>SMKPRCLHLEKGPQGFGFLLREEKGLDGRPGQFLWEVDPGLPAKKAGMQAGDRLVAVAGESVEGLGHEETVSRIQGQGSCVSLTVVDPEADRETSV[6x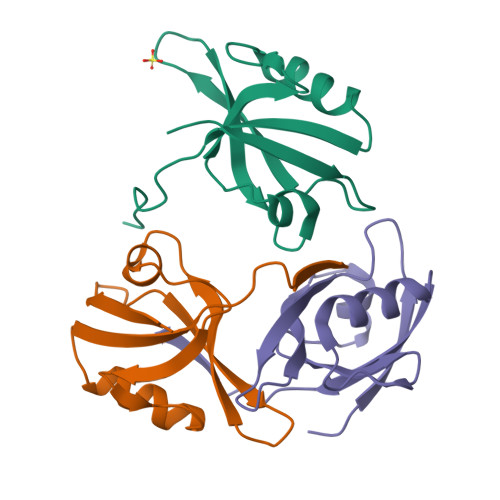]> MDLTVEPNLHSLITSTTHKWIFVGGKGGVGKTTSSCSIAIQMALSQPNKQFLLISTDPAHNLSDAFGEKFGKDARKVTGMNNLSCMEIDPSAALKDMNDMAVSRANNNGSDGQGDDLGSLLQGGALADLTGSIPGIDEALSFMEVM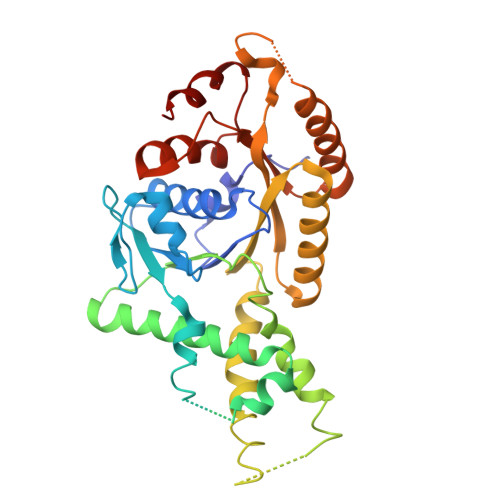KHIKRQEQDEGETFDTVIFDTAPTGHTLRFLQLPNTLSKLLEKFGEITNKLGPMLNSFMGAGNVDISGKLNELKANVETIRQQFTDPDLTTFVCVCISEFLSLYETERLIQELISYDMDVNSIIVNQLLFAENDQEHNCKRCQARWKMQKKYLDQIDELYEDFHVVKMPLCAGEIRGLNNLTKFSQFLNKEYNPITDGKVIYELEDKE> MAHHHHHHMEKVRVRFAPSPTGPLHLGGVRTALYDYLFAKHNGGDFILRIEDTDTQRYVPGSEEYIMEALEWIGMVPDESPKHGGPYAPYRQSERRDIYDRYTEQILKTDYAYLAFDTPEELDQIRAEFEARGDVFAYNYETRNRLRNSISLPEEEVKKLLEEKTPYVIRFKMPLDRIINLNDIIRGKFSVNTNTL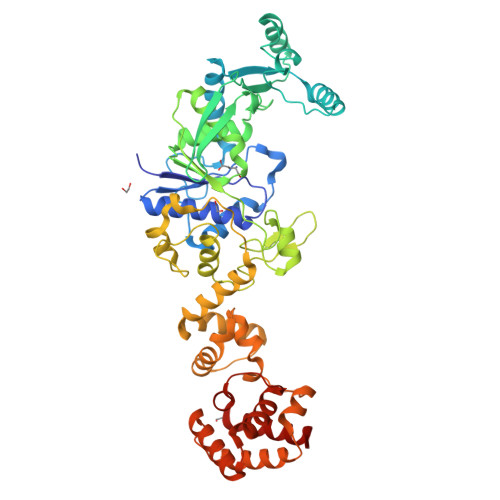DDKVLVKNDGMPTYHFANIIDDHEMKITHVIRGEEWLPSMALHVLLYEAMGWDAPEFAHLSLILKPEGKGKLSKRDGDKFGFPVFPLNFTDSATGNTSAGYREEGYLPEAFINMVAMLGWSPADNKEIVSMDEMIKEFDLNKVHKAGARFSAEKAKWFNQQYLQLMSNEAILPEFKKVLAENNVEVSDEKALKIIGLMKERATFVKDIYNDGKFFFHAPESFDEKASKKAWSPETAVLMQELTEAISSLDFKAEIIKESIHHLAEAKGLGMGKVMMPLRLSLVGELKGPDVPDLMEMIGKEETISRINKAIETLK> SEQETRGANEAIDFNDELRNRREKLAALRQQGVAFPNDFRRDHTSDQLHEEFDAKDNQELESLNIEVSVAGRMMTRRIMGKASFVTLQDVGGRIQLYVARDSLP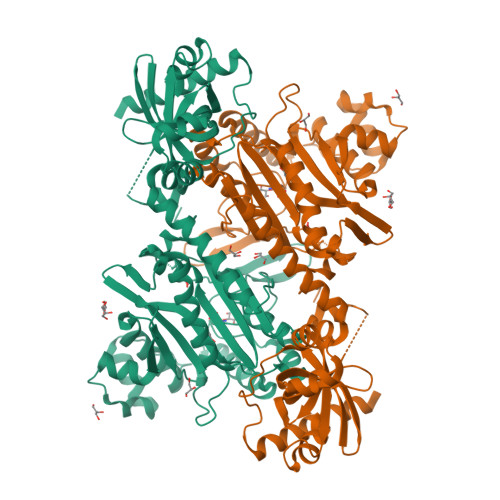EGVYNDQFKKWDLGDIIGARGTLFKTQTGELSIHCTELRLLTKALRPLPDKFHGLQDQEVRYRQRYLDLIANDKSRQTFVVRSKILAAIRQFMVARGFMEVETPMMQVIPGGASARPFITHHNALDLDMYLRIAPELYLKRLVVGGFERVFEINRNFRNEGISVRHNPEFTMMELYMAYADYHDLIELTESLFRTLAQEVLGTTKVTYGEHVFDFGKPFEKLTMREAIKKYRPETDMADLDNFDAAKALAESIGITVEKSWGLGRIVTEIFDEVAEAHLIQPTFITEYPAEVSPLARRNDVNPEITDRFEFFIGGREIGNGFSELNDAEDQAERFQEQVNAKAAGDDEAMFYDEDYVTALEYGLPPTAGLGIGIDRMIMLFTNSHTIRDVILFPAMRPQK> GSHMLDFRVEYRDRNVDVVLEDTCT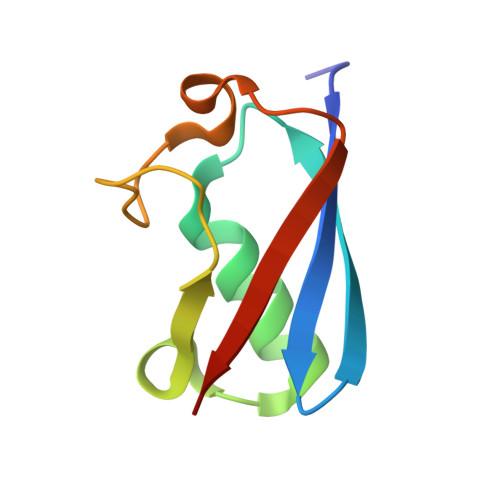VGEIKQILENELQIPVSKMLLKGWKTGDVEDSTVLKSLHLPKNNSLYVLTPDL>[4x]EVAAVVVVGSCMTDLVSLTSRLPKTGETIHGHKFFIGFGGKGANQCVQAARLGAMTSMVCKVGKDSFGNDYIENLKQNDISTEFTYQTKDAATGTASIIVNNEGQNIIVIVAGANLLLNTEDLRAAANVISRAKVMVCQLEITPATSLEALTMA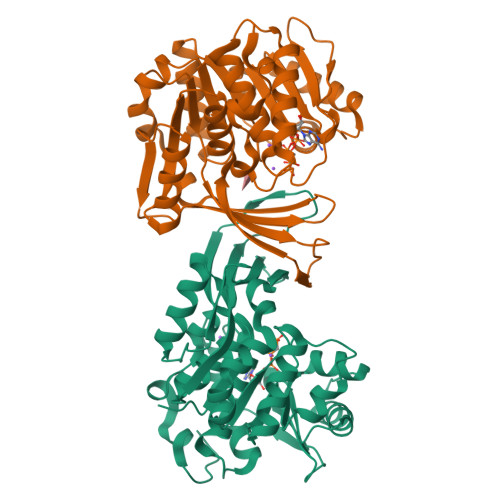RRSGVKTLFNPAPAIADLDPQFYTLSDVFCCNESEAEILTGLTVGSAADAGEAALVLLKRGCQVVIITLGAEGCVVLSQTEPEPKHIPTEKVKAVDTTGAGDSFVGALAFYLAYYPNLSLEDMLNRSNFIAAVSVQAAGTQSSYPYKKDLPLTLFLEHHHHHH>MSLHDFTLADVYRRNAALFPDRTAFMVDGVRLTHRDYLARAERLASGLLRDGVHTGDRVAILSQNCS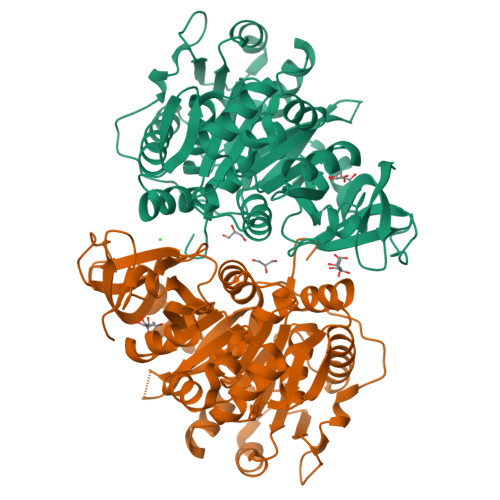EMIELIGAVALIGAILLPVNYRLNADEIAFVLGDGAPSVVVAGTDYRDIVAGVLPSLGGVKKAYAIGDGSGPFAPFKDLASDTPFSAPEFGAADGFVIIHTAAVGGRPRGALISQGNLLIAQSSLVDAWRLTEADVNLGMLPLFHVTGLGLMLTLQQAGGASVIAAKFDPAQAARDIEAHKVTVMAEFAPMLGNILDQAAPAQLASLRAVTGLDTPETIERFEATCPNATFWATFGQSETSGLSTFAPYRDRPKSAGRPLFWRTVAVVDAEDRPLPPGEVGEIVLRGPTVFKGYWNNAAATQHAFRNGWHHTGDMGRFDADGYLFYAGRAPEKELIKTGGENVYPAEVEGALKQHPAIADAVVIGVPDPQWSEAIKAVCVCKPGESIAADALAEFVASLIARYKKPKHVVFVEALPKDAKGAIDRAAVKTAHGQEGHHHHHH[2x]>[24x]VESSTDGQVVPQEVLNLPLEKAHEEADDYLDHLLDSLEELSEAHPDCIPDVELSHGVMTLEIPAFGTYVINKQPPNKQIWLASPLSGPNRFDLLNGE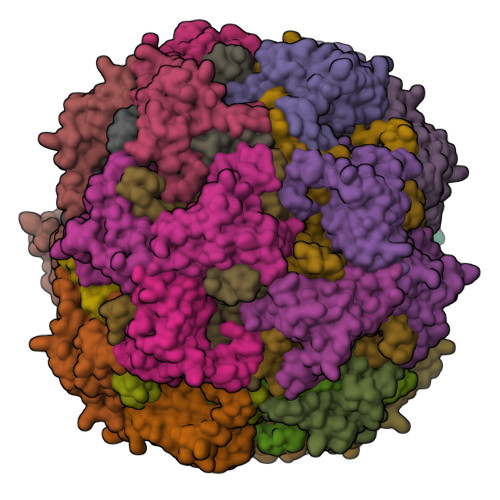WVSLRNGTKLTDILTEEVEKAISK;>GSHMSSITKRLYHPKVIEHYTHPRNVGSLDKKLPNVGTGLVGAPACGDVMRLQIKVNDSTGVIEDVKFKTFGCGSAIASSSYMTELVQGMTLDDAAKIKNTEIAKELSLPPVKLHCSMLAEDAIKAAIKDYKSKRNTPTMLS[24x]> MKTITETLNLAPKGKNFLTADWPAPANVKTLITTRNGGVSQGAYQSLNLGTHVGDNPEAVRRNREIVQQQVGLPVAYLNQIHSTVVVNAAEALGGTPDADASVDDTGKVACAVMTADCLPVLFCDRAGTAVAAAHAGWRGLAGGVLQNTIAAMKVPPVEMMAYLGPAISADAFEVGQDVFDAFCTPMPEAATAFEGIGSGKFLADLYALARLILKREGVGGVYGGTHCTVLE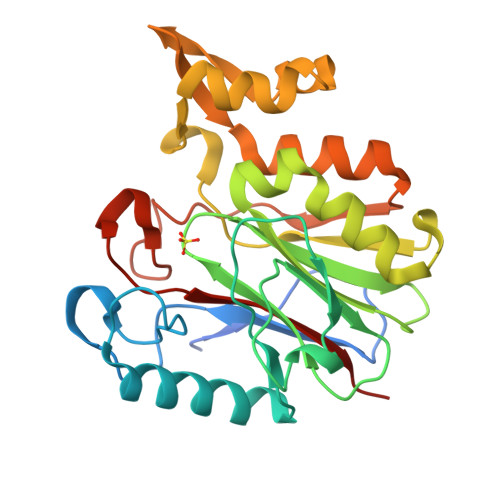RDTFFSYRRDGATGRMASLIWLDGNAV4-[(4-fluoro-2-methyl-3H-indol-5-yl)oxy]-6-methoxy-7-[3-(pyrrolidin-1-yl)propoxy]quinazoline | C25 H27 F N4 O3 | 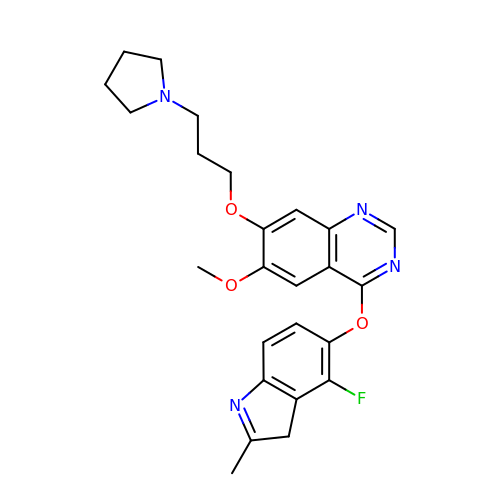ZOVVOYNGCNKFNN-UHFFFAOYSA-N> INIDDILAELDKETTAVDSTKITQGSSSTTHRDANTIVGSSLDLNDKTQIYVSPQQDFSDLMKSWKNERCSPELLPYPHQLMKRLLNRISMQSQLIENISMGFLDMQNASNANPPMPNESKLPLLCMETELERLKFVIRSYIRCRLSKIDKFSLYLRQLNEDENSLISLTDLLSKDEIKYHDTHSLIWLKLVNDSILKYMPEELQAINDTEGSVNMIDEPDWNKFVFIHVNGP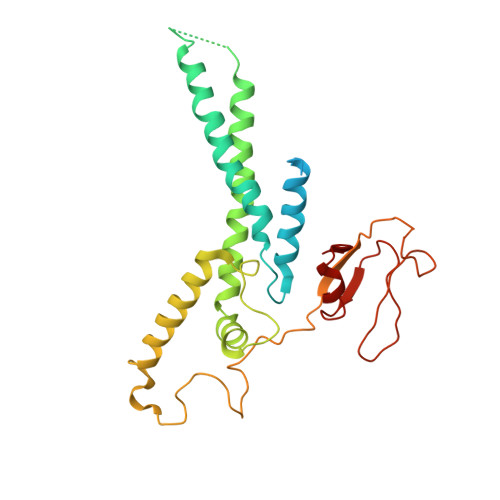PDGKWNEDPLLQENEFGKPCYTVTIPDLKEEVELTIGSIYVMRYEVIRDLLRDDKVAL>MPKSFYDAVGGAKTFDAIVSRFYAQVAEDEVLRRVYPEDDLAGAEERLRMFLEQYWGGPRTYSEQRGHPRLRMRHAPFRISLIERDAWLRCMHTAVASIDSETLDDEHR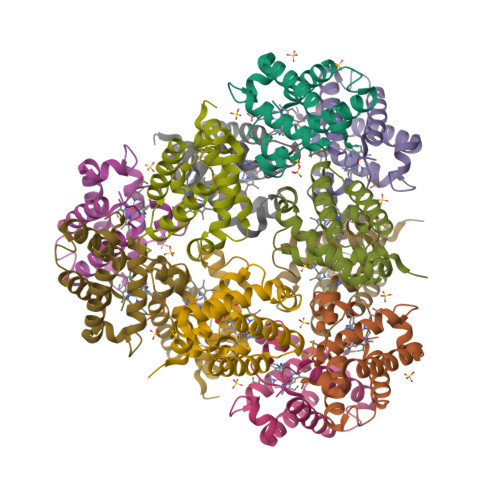RELLDYLEMAAHSLVNSPF[12x]> GAMGYKDNIRHGVCWIYYPDGGSLVGEVNEDGEMTGEKIAYVYPDERTALYGKFIDGEMIEGKLATLMSTEEGRPHFELMPGNSVYHFDKSTSSCISTNALLPDPYESERVYVAESLISSAGEGLFSKVAVGPNTVMSFANGVRITHQEVDSRDWALNGNTLSLDEETVIDVPEPYNHVSKYCASLGHKANHSFTPNCIYDMFVHPR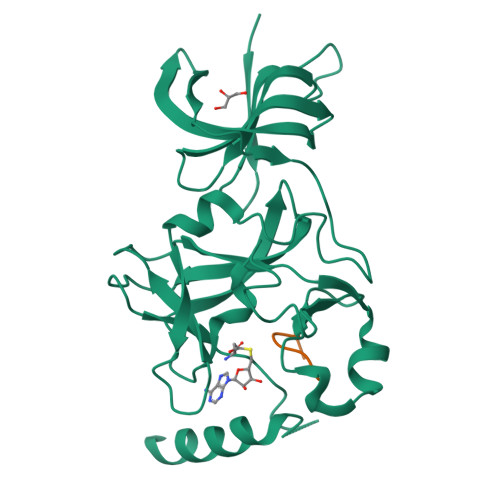FGPIKCIRTLRAVEADEELTVAYGYDHSPPGKSGPEAPEWYQVELKAFQATQQK;> XSKSKDRKYTL> SLPFTFKVP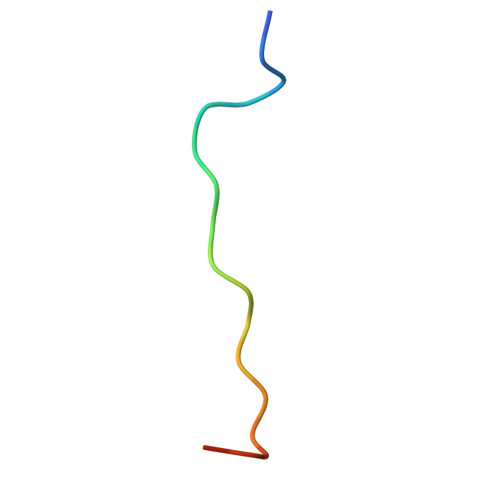APPPSLPPSW>[2x]HMPAPKTIYIAGPAVFHPDNGEAYYNNVRALMKGKDVVPLIPTDNIATGAVNIRNKNIDMIRACDAIIADLSPFRSKEPDCGTAFELGYAAALGKVLL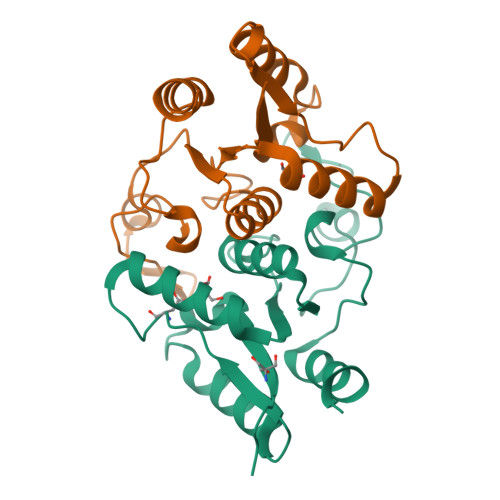TFSTDTRPMVEKYGSEMADGLSVENFGLPFNLMLHDGTDVFDSFEAAFAYFVEHHLTP N~3~-(3-PYRIDIN-3-YLBENZYL)PYRIDINE-2,3-DIAMINE 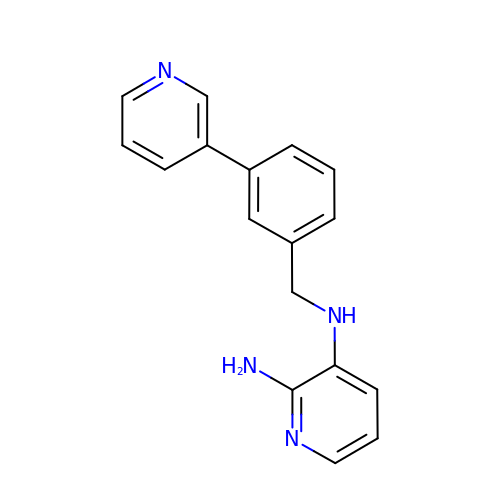| C17 H16 N4 | NQSBHBFOOVYRNM-UHFFFAOYSA-N>[2x]MQPARAATWRDEIRAIAFDVQGTCVDFYQPILRAGQTVNAAKGLALDWAKLSGEWRDLYRVALDEVIAGKRPWIRVDRIYREALDVLLDRHGLSEAFSKDERDELNTVWSKLDAWPDSVEGLARLRSRFVTSTLSNAGMAAVVAVVKHAGLPFDALLTAELAHSYKPSPAVYQLAVDYLGYPADTILMVACHKYDLKAARAFGMRTAFVARPLEFGPAAKVDVAPESWFDLHVDNFTQLADALVPALEHH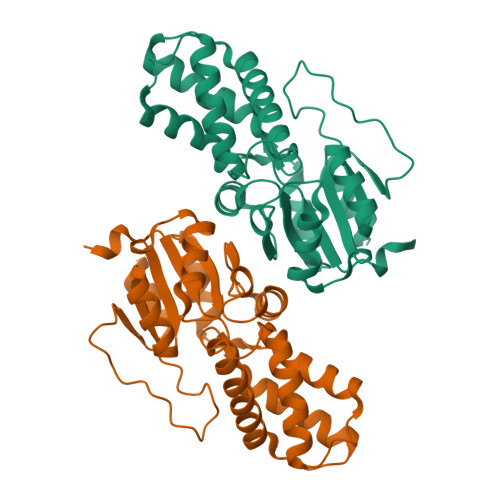HHHH> FQGMKLLVVYDVSDDSKRNKLANNLKKLGLERIQRSAFEGDMDSQRM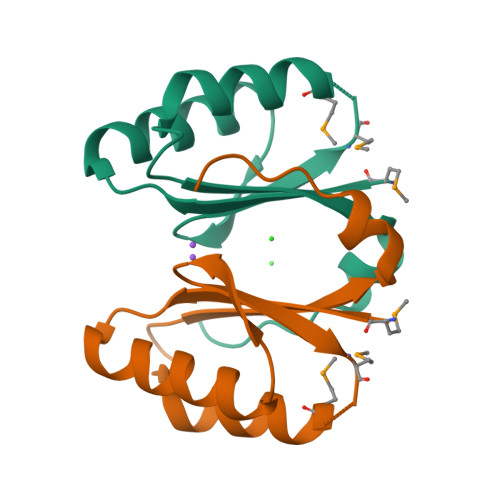KDLVRVVKLIVDTNTDIVHIIPLGIRDWERRIVIGREGLEEWLV> GAMAMRIYYIGVFRSGGEKALELSEVKDLSQFGFFERSSVGQFMTFFAETVASRTGAGQRQSIEEGNYIG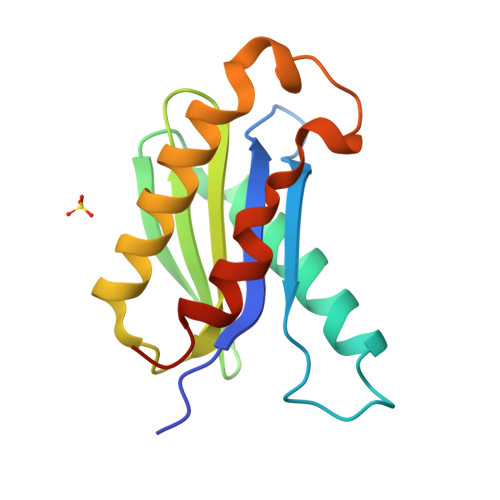HVYARSEGICGVLITDKEYPVRPAYTLLNKILDEYLVAHPKEEWADVTETNDALKMKQLDTYISKYQDPSQADA> SGQEFLVFTLG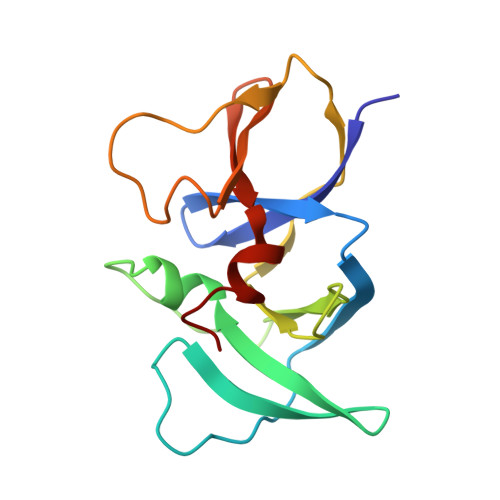DEEYGIDILKVQEIRGYDQVTRIANTPAFIKGVTNLRGVIVPIVDLRIKFSQVDVDYNDNTVVIVLNLGQRVVGIVVDGVSDVLSLTAEQIRPAPEFAVTLSTEYLTGLGALGDRMLILVNIEKLLNSEEMA> GAMAEYEIDEITFHKRLGILLTSWKNEEDGKTLFQDCDSILVTVGAHDDTNPYQKSTALHTWLLGYEFPSTLILLEKHRITILTSVNKANMLTKLAETKGAAADVNILKRTKDAEENKKLFEKIIEY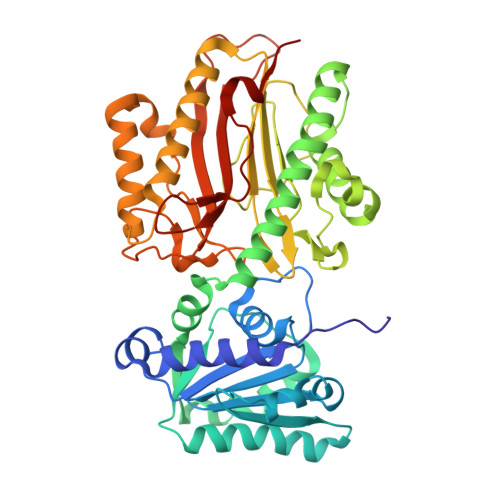IRATNKKVGVFPKDKTQGKFINEWDSIFEPVKSEFNLVDASLGLAKCLAIKDEQELANIKGASRVSVAVMSKYFVDELSTYIDQGKKITHSKFSDQMESLIDNEAFFQTKSLKLGDIDLDQLEWCYTPIIQSGGSYDLKPSAITDDRNLHGDVVLCSLGFRYKSYCSNVGRTYLFDPDSEQQKNYSFLVALQKKLFEYCRDGAVIGDIYTKILGLIRAKRPDLEPNFVRNLGAGIGIEFRESSLLVNAKNPRVLQAGMTLNLSIGFGNLINPHPKNSQSKEYALLLIDTIQITRSDPIVFTDSPKAQGDISYFFGED> MKLNKQNLTQLAPEVKLPAYTLADTRQGIAHIGVGGFHRAHQAYYTDALMNTGEGLDWSICGVGLRSEDRKARDDLAGQDYLFTLYELGDTDDTEVRVIGSISDMLLAEDSAQALIDKLASPEIRIVSLTITEGGYCIDDSNGEFMAHLPQIQHDLAHPSSPKTVFGFICAALTQRRAAGIPAFTVMSCDNLPHNGAVTRKALLAFAALHNAELHDWIKAHVSFPNAMVDRITPMTSTAHRLQLHDEHGIDDAWPVVCEPFVQWVLEDKFVNGRPAWEKVGVQFTD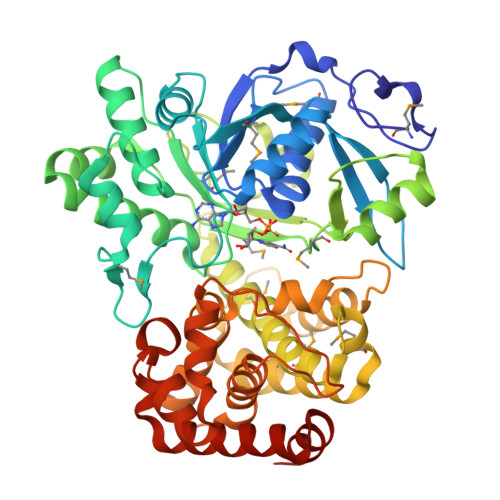DVTPYEEMKIGLLNGSHLALTYLGFLKGYRFVHETMNDPLFVAYMRAYMDLDVTPNLAPVPGIDLTDYKQTLVDRFSNQAIADQLERVCSDGSSKFPKFTVPTINRLIADGRETERAALVVAAWALYLKGVDENGVSYTIPDPRAEFCQGLVSDDALISQRLLAVEEIFGTAIPNSPEFVAAFERCYGSLRDNGVTTTLKHLLKKPV> ATLDVRGGYRSGSHAYETRLKVSEGWQNGWWASMESNTWNTIHDNKKENAALNDVQVEVNYAIKLDDQWTVRPGMLTHFSSNGTRYGPYVKLSWDATKDLNFGIRYRYDWKAYRQQDLSGDMSRDNVHRWDGYVTYHINSDFT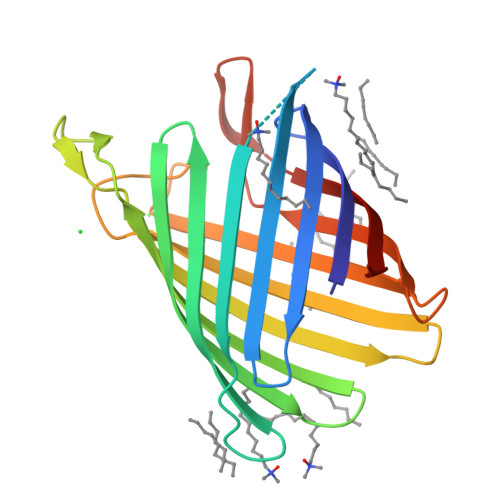FAWQTTLYSKQNDYRYANHKKWATENAFVLQYHMTPDITPYIEYDYLDRQGVYNGRDNLSENSYRIGVSFKL In this work, we exhaustively probe the ability of all 36 immobile HJ sequences to form DNA crystals in two different designed systems. Three separate self-assembling DNA crystal systems are described in this report: the “4 × 5” and “4 × 6” designs (collectively referred to as the 4 × N systems), and a third construct with a “scrambled” sequence variant of the 4 × 6 lattices. Self-assembly was mediated by three constituent oligonucleotides: (S1) containing four sequence repeats of either 5 or 6 bases; (S2) composed of 21 bases containing complementary regions to both (S1); and (S3) which forms the second junction crossover. The HJ serves as the fundamental component at the core of each unit, and the ultimate assembly of the full lattice is facilitated by the complementary 2-base sticky ends that tail each duplex.

In parallel, we employed the previously reported J1 4 × 6 system (3.05 Å), with P32 symmetry. Seventeen of the 36 junctions successfully crystallized, a 47% success rate. Unlike the 4 × 5 motif, nearly all of the 4 × 6 junction sequences had a strong preference for crystallization in buffers containing ≥2.0 M salts (e.g., LiCl, Li2SO4, KCl, and NaCl), with the majority preferring slightly basic pH conditions in cacodylic acid. The average cell constants for the P32 crystals were a = b = 68.29 Å c = 55.68 Å. The c-axis, in particular, was ~5 Å shorter, and had a much larger degree of variability (σ = 1.97), than those that crystallized using the 4 × 5 motif. The broad range of the short axis spanned from 52.77 to 60.36 Å, and we posit that the flexible axis lengths could be responsible for rendering a larger number of junctions fatal than the 4 × 5 system. The average junction angles of 54.60° (σ = 1.44) and 58.37° (σ = 2.3) for the P32 and R3 symmetries, respectively, along with their preference for salts or organic solvents, were likely the major contributing factors that yielded the divergent lattices. However, in the majority of the crystal structures reported here, the cacodylate anion indeed fits best into the electron density map of our X-ray structures, due to the presence of sodium cacodylate in the crystallization solution.

> GAGCAGACTTGA;> CGACACTCA;> TCATCG;> TCTGAGTAGGTCTGC> MNAVEIQGVSQRYGSMTVLHDLNLNLGEGEVLGLFGHNGAGKTTSMKLILGLLSPSEGQVKVLGRAPNDPQVRRQLGYLPENVTFYPQLSGRETLRHFARLKGAALTQVDELLEQVGLAHAADRRVKTYSKGMRQRLGLAQALL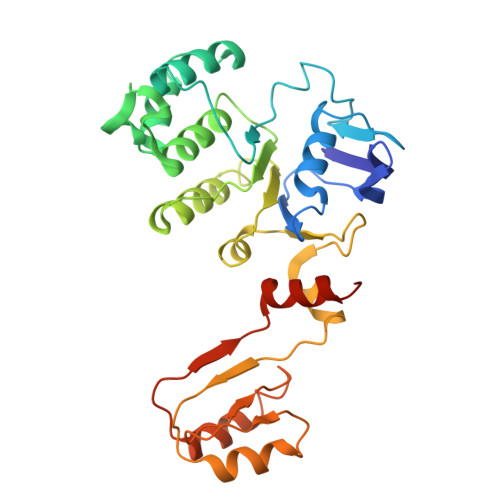GEPRLLLLDQPTVGLDPIATQDLYLLIDRLRQRGTSIILCSHVLPGVEAHINRAAILAKGCLQAVGSLSQLRAEAGLPVRIRASGISERDSWLQRWTDAGHSARGLSESSIEVVAVNGHKLVLLRQLLGEGEPEDIEIHQPSLEDLYRYYMERAGDVRAQEGRL{(1R,2R)-2-[4-(carboxymethyl)benzene-1-carbonyl]cyclopentyl}propanedioic acid | 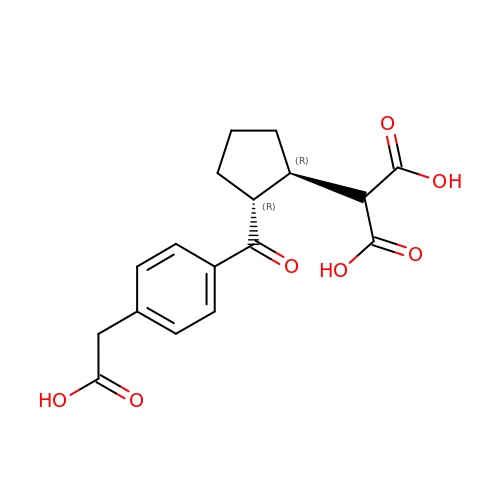C17 H18 O7 | HXTDFADOGPNOAK-VXGBXAGGSA-N> MSEAEARPTNFIRQIIDEDLASGKHTTVHTRFPPEPNGYLHIGHAKSICLNFGIAQDYKGQCNLRFDDTNPVKEDIEYVESIKNDVEWLGFHWSGNVRYSSDYFDQLHAYAIELINKGLAYVDELTPEQIREYRGTLTQPGKNSPYRDRSVEENLALFEKMRAGGFEEGKACLRAKIDMASPFIVMRDPVLYRIKFAEHHQTGNKWCIYPMYDFTHCISDALEGITHSLCTLEFQDNRRLYDW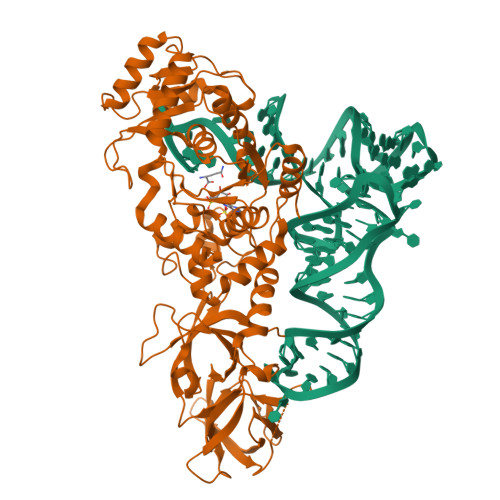VLDNITIPVHPRQYEFSRLNLEYTVMSKRKLNLLVTDKHVEGWDDPRMPTISGLRRRGYTAASIREFCKRIGVTKQDNTIEMASLESCIREDLNENAPRAMAVIDPVKLVIENYQGEGEMVTMPNHPNKPEMGSRQVPFSGEIWIDRADFREEANKQYKRLVLGKEVRLRNAYVIKAERVEKDAEGNITTIFCTYDADTLSKDPADGRKVKGVIHWVSAAHALPVEIRLYDRLFSVPNPGAADDFLSVINPESLVIKQGFAEPSLKDAVAGKAFQFEREGYFCLDSRHSTAEKPVFNRTVGLRDTWAKVGE>MKKVIIAGNGPSLKEIDYSRLPNDFDVFRCNQFYFEDKYYLGKKCKAVFYNPSLFFEQYYTLKHLIQNQEYETELIMCSN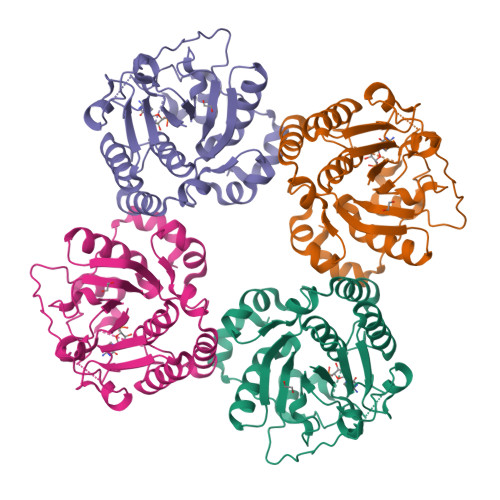FNQAHLENENFVKTFYDYFPDAHLGYDFFKQLKDFNAYFKFHEIYFNQRITSGVYMCAVAIALGYKEIYLSGIDFYQNGSSYAFDTKQKNLLKLAPNFKNDNSHYIGHSKNTDIKALEFLEKTYKIKLYCLCPNSLLANFIGLAPNLNSNFIIQEKNNYTKDILIPSSEAYGKFSKNIN[2x]VhCBP is a periplasmic chitooligosaccharide-binding protein mainly responsible for translocation of the chitooligosaccharide (GlcNAc)2 across the double membranes of marine bacteria. The chitooligosaccharide-specific SBP is localized to the periplasmic compartment of the bacterial cell wall and serves as a mobile component of the (GlcNAc)2-specific ABC transporter. SBPs share a common structural feature comprising two domains connected by a flexible hinge region. VcCBP and VhCBP belong to cluster C/subcluster IV (C-IV), members of which are specific for oligosaccharides, including mannooligosaccharides, cellooligosaccharides, and chitooligosaccharides.

(GlcNAc)4 partially occupied the closed sugar-binding groove, with two reducing-end GlcNAc units extending beyond the sugar-binding groove and barely characterized by weak electron density. The electron density of (GlcNAc)4 on the reducing-end side was too weak to place the two GlcNAc moieties at the imaginary affinity sites 3 and 4. This suggests that the mobility of the fourth sugar has a knock-on effect to weaken the binding of the third sugar. Flipping of the Phe411 side chain was also observed in the complex with (GlcNAc)4, as in the complex with (GlcNAc)3, and appears to widen the space at sites 3 and 4. It is most likely that GlcNAc residues are present at sites 3 and 4 and are disordered because of the large space on these two sites. Docking simulation of the structure of VhCBP in complex with (GlcNAc)4 revealed that interactions are formed mostly with the two GlcNAc units at the affinity sites 1 and 2, whereas on sites 3 and 4, only two hydrogen bonds are formed, by the main-chain carbonyl of Ala514 and the Oδ side chain of Gln102, respectively. The middle glycosidic linkage of the bound (GlcNAc)4 was also twisted, as in (GlcNAc)3 bound to VhCBP. The disadvantage derived from the twist of the glycosidic linkage appears to predominate over the advantages derived from additional interactions/disorder of the GlcNAc residues at sites 3 and 4, resulting in the lower affinity for (GlcNAc)4. The binding affinity did not correspond to the degree of polymerization and was the lowest in the longest ligand, (GlcNAc)4.

> AERSELTIHPKEFTTFVRNFNPFLGATNLHTTTDFIYEPLVVFNEMHGNTPVFRLAENFQMSDDLMSVTFDIRKGVKWSDGEAFTADDVVYSFNLVKEKPELDQSGINSWVTGVEKVNDYQVKFRLSEANSNVPYEIAKVPVVPKHVWSKVKDPSTFTNENPVGSGPFTVIDTFTPQLYIQCENPNYWDAANLDVDCLRVPQIANNDQFLGKVVNGEMDWTSSFVPDIDRTYAAASPKHHYWYPPAGTQAFVVNFKNPDAAKNEALTNVDFRRAFSMALDRQTIIDIAFYGGGTVNDFASGLGYAFEAWSDEKTHDKFKAYNSYNAEGAKKLLAKAGFKDVNKDGFVDTPSGKSFELLIQSPNGWTDFNNTVQLAVEQLAEVGIKARARTPDFSVYNQAMLEGTYDVAYTNYFHGADPYTYWNSAYNSALQSGDGMPRFAMHFYKNEKLDGLLNSFYKTADKQEQLEIAHGIQQIIAQDQVTIPVLSGAYMYQYNTTRFTGWWNEENPKGRPNIWAGIPERLLHVLDLKPVKLEHHHHHH> MYKKALHSFFLKVHPDFFHHNRSQQTVNESSVARLNELLSWAKAFKSGHLQPPPSSSFTLTFYRKPDDNMGNGETRREGSGSPVSSLVGRSMGDGSLSPTIIQSTFELPSNFAPSDNHRGTVERAVNKFLRDLLRRAACIDSVTESISEAEDATAARAEAKPLRRRPRGSQHRGAPTGPKSLLDEAVESMTVQWSLTPAPTLQELIEADQILFSRDLSPLQSAAALSTLQRHLGELNYSAWESMPVIVSNQFSIGDLTGTITIPWDFTPEQFHSFMAHNEKGVARCREVAIQYASTIEQLIAELCTA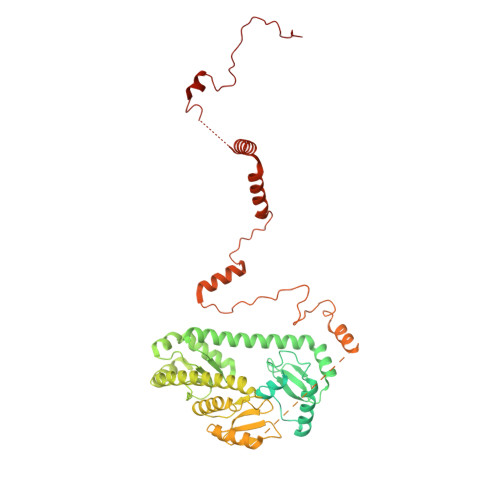LELDDILVSCSHQDALRLMELLHRNRELLIQYGLSKLTLEVGNRHATRANGVVIINCSLTSEQLRPWLKAISPKLPLQQRLYELSKQMLESTLWHLKEFRTMVEPGGVDAFSNDCTYAERLQWSKELFRIGPSLAPWDWSEMTFVLSPDVDIDWANGLLALPYNFDGDALVRYVEEVQQEAKSRKREELLAASAMQREEEERRRKQQHDEELMVECQEKGERSGDDSPTVAERMRHLYRQTNPHMDEYLASSNSRVDTLPVERPLSHAVTFNSDAEAEDQLKWEGFYAEPYVDQAPTSDIDDMAHTFMLTNRWHREEAAKKMLDQLRGTYGKKSRRFEYQKMGDVLEINNAKVQPKGFPTLTRGIKPGC>MDIISVALKRHSTKAFDASKKLTAEEAEKIKTLLQYSPSSTNSQPWHFIVASTEEGKARVAKSAAGTYVFNERKMLDASHVVVFCAKTAMDDAWLERVVDQEEADG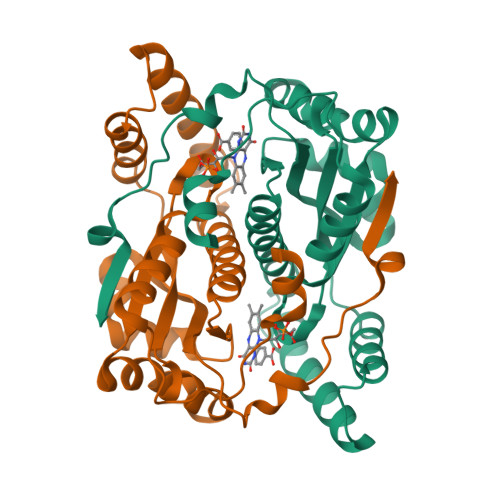RFNTPEAKAANHKGRTYFADMHRVDLKDDDQWMAKQVYLNVGNFLLGVGAMGLDAVPIEGFDAAILDEEFGLKEKGFTSLVVVPVGHHSVEDFNATLPKSRLPLSTIVTEC[4x]>[2x]MDWLLTPGPVRLHPKALEALARPQLHHRTEAAREVFLKARGLL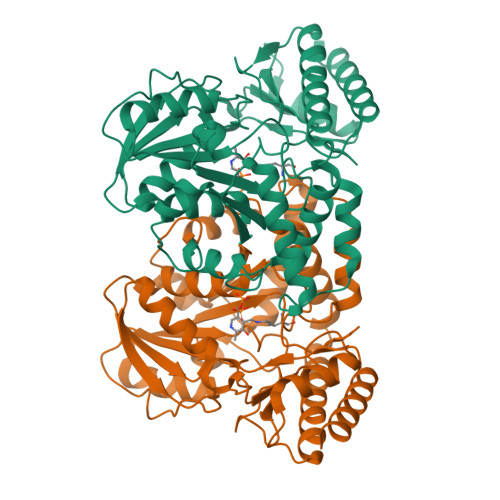REAFRTEGEVLILTGSGTLAMEALVKNLFAPGERVLVPVYGKFSERFYEIALEAGLVVERLDYPYGDTPRPEDVAKEGYAGLLLVHSETSTGALADLPALARAFKEKNPEGLVGADMVTSLLVGEVALEAMGVDAAASGSQKGLMCPPGLGFVALSPRALERLKPRGYYLDLARELKAQKEGESAWTPAINLVLAVAAVLEEVLPRLEEHLALKAWQNALLYGVGEEGGLRPVPKRFSPAVAAFYLPEGVPYARVKEAFAQRGAVIAGGQGPLKGKVFRLSLMGAYDRYEALGVAGMFREVLEEILPAS>[2x]EQQVPILEKFCFTPHTEEGCLSERAALQEELQLCKGLVQA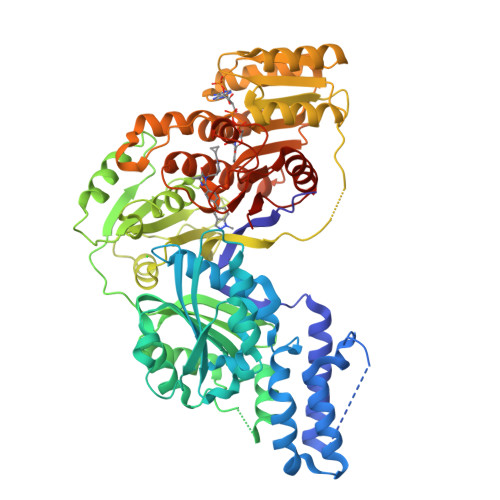LQTKVTQQGLKMVVPGLDGAQIPRDPSQQELPRLLSAACRLQLNGNLQLELAQVLAQERPKLPEDPLLSGLLDSPALKACLDTAVENMPSLKMKVVEVLAGHGHLYSRIPGLLSPHPLLQLSYTATDRHPQALEAAQAELQQHDVAQGQWDPADPAPSALGSADLLVCNCAVAALGDPASALSNMVAALREGGFLLLHTLLRGHPLGDIVAFLTSTEPQYGQGILSQDAWESLFSRVSLRLVGLKKSFYGSTLFLCRRPTPQDSPIFLPVDDTSFRWVESLKGILADEDSSRPVWLKAINCATSGVVGLVNCLRREPGGNRLRCVLLSNLSSTSHVPEVDPGSAELQKVLQGDLVMNVYRDGAWGAFRHFLLEEDKGGSKTGCPAHKSYIIAGGLGGFGLELAQWLIQRGVQKLVLTSRSGIRTGYQAKQVRRWRRQGVQVQVSTSNISSLEGARGLIAEAAQLGPVGGVFNLAVVLRDGLLENQTPEFFQDVCKPKYSGTLNLDRVTREACPELDYFVVFSSVSCGRGNAGQSNYGFANSAMERICEKRRHEGLPGLAVQWGAIGDVGILVETMSTNDTIVSGTLPQRMASCLEVLDLFLNQPHMVLSSFVLAEKAAAYRDRD>[4x]MRGSHHHHHHGSVTTKRYTL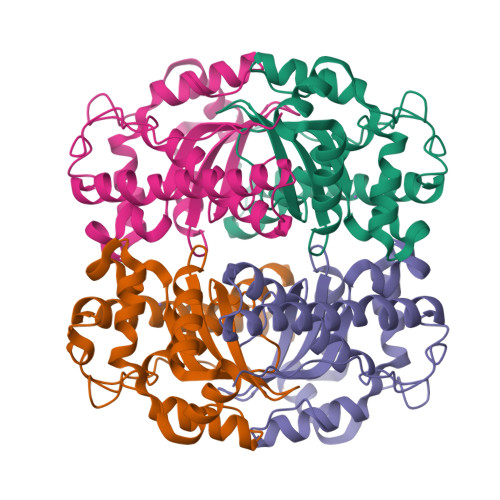PPLPYAYNALEPYISAEIMQLHHQKHHQGYVNGANAALEKLEKFRKGEAQIDIRAVLRDLSFHLNGHILHSIFWPNMAPPGKGGGKPGGKIADLINKFFGSFEKFKEEFSQAAKNVEGVGWAILVYEPLEEQLLILQIEKHNLMHAADAQVLLALDVWEHAYYLQYKNDRGSYVDNWWNVVNWDDVERRLQKALNGQIALKL>MHHHHHHHHHHHHLPPITPQELESMSPQEQRAALGDRLFLKVYEIAPELAPKITGMFLEMKPKEAYELLNDQKRLEERVTEALCVLKAHQTA[2x]

NMR and X-ray crystallography reveal that Leishmania has a unique type of N-terminally-extended cap-binding protein (eIF4E4) that binds via a PAM2 motif to PABP1. Exceptionally, therefore, by binding tightly to two protein ligands and to the mRNA 5′ cap4 structure, the trypanosomatid N-terminally extended form of eIF4E acts as the core molecular scaffold for the mRNA-cap-binding complex. Thus, in Leishmania, the chain of interactions 5′cap4-eIF4E4–PABP1-poly(A) bridges the mRNA 5′ and 3′ ends. Finally, the eIF4E4 N-terminal extension is an intrinsically disordered region that transitions to a partly folded form upon binding to PABP1, whereby this interaction is not modulated by poly(A) binding to PABP1.

In further work, we were able to solve the crystal structures of PABP1(J) and of PABP1(J) co-crystallized with a synthetic eIF4E4 PAM2 peptide, both to a resolution of ∼2 Å. Obtaining these structures enabled us to locate the binding motif for eIF4E4 in relation to the three-dimensional structure of Leishmania PABP1. Consistent with the structures of other analogous complexes, binding is associated with relatively minor changes in the conformation of the PABP1 fragment; the side chains of only Lys 520 and Glu 527 are affected. Our results suggest that the changes in the roles of the respective translation factors in Leishmania have created a biomolecular chain that functions without poly(A)-mediated modulation of protein-protein interactions. This outcome is consistent with the observation that the PABP1 PABC domain forms a stable fold in solution that is only minimally altered by binding of the eIF4E4 peptide. The 1H–15N-HSQC NMR spectra showed PABP1(J) to be folded, while eIF4E4(iv) displayed amide resonance chemical shift dispersion characteristic of an intrinsically disordered domain.> SMSGISPKKSKYMTPMQQKLNEVYEAVKNYTDKRGRRLSAIFLRLPSRSELPDYYLTIKKPMDM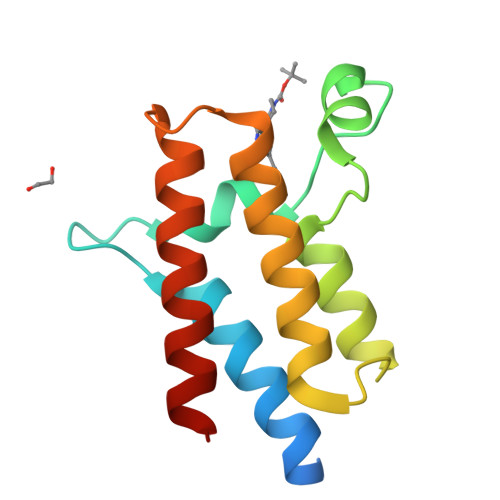EKIRSHMMANKYQDIDSMVEDFVMMFNNACTYNEPESLIYKDALVLHKVLLETRRDLEGD>[4x]MDFLDSLIWERVVDDQYVTNPTFCISDYFEIVRQPGDGNCFYHSIAELFFDVKTPFSFRKVKEHLRLAADAFYDTEPEAIGTGVTKEEYIQAAMKDNEWGGSLEASMLSKQLQITIILWVVNQTEQVTAAIKFGPGRVSTALNLMHVGRTHFDALRVINQLEDNQLQSRSGSHHHHHH;>MATLNILVRNDKGRSSSYEVQLTQTVAVLKQQVCQRERVQADQFWLSFEGKPMDDEHPLGEYGLTTGCTVFMNLRLRG[4x]

Beyond the RNA-dependent RNA polymerase (RdRp), the L protein contains a viral homologue of the ovarian tumor domain protease (OTU) at the N-terminus. This OTU reverses posttranslational modifications by ubiquitin (Ub) and interferon (IFN) stimulated gene product 15 (ISG15). Sheep ISG15 was derivatized into a suicide inhibitor with propargylamine and incubated with KUPEV and GANV OTUs to form covalent complexes that could be used for X-ray crystallography. This yielded an atomic resolution structure of KUPEV OTU bound to the C-terminal domain of sheep ISG15 (C-sheep ISG15) solved to 2.06 Å and a low-resolution structure of GANV OTU bound to full length sheep ISG15 to 3.15 Å.

Examination of the high resolution KUPEV and low resolution GANV OTU-sheep ISG15 structures reveals them to possess the familiar overall mode of OTU-substrate binding, in which the OTU binds to the C-terminal domain of ISG15 by a mix of hydrophobic and electrostatic interactions. On the sheep ISG15 side, the interface with the OTUs is formed by W123, P130, and F149. One of the most noteworthy interactions is that of sheep ISG15 D89 forming water-mediated interactions with both KUPEV OTU T128 and R149. Interestingly, this results in D89 pointing away from the interface, contrasting with previous observations for this residue position in OTU-Ub structures and CCHFV OTU-human ISG15 structures. Considering the selectivity pocket in KUPEV is lined by hydrophobic residues V18, V120, A129, and I131, the adoption of a more solvent-exposed confirmation of the charged aspartate in sheep ISG15 is understandable. For instance, the OTUs from KUPEV and DUGV have limited activity for human proISG15, but efficiently cleave sheep and cow proISG15s and show moderate activity towards camel and vesper bat proISG15s. In the KUPEV OTU residue 122 is an asparagine residue, while CCHFV is unique among OTUs with an alanine at this position. As anticipated, the GANV OTU E122N mutant reduced activity for human ISG15-AMC almost 10-fold, while KUPEV OTU N122E boosted activity more than 6-fold relative to WT. In KUPEV OTU this residue is an isoleucine, creating the potential for a steric clash with the longer glutamate in human ISG15 compared to aspartate in sheep ISG15. In contrast, the KUPEV helix mutant (I80R/G81L/T82V) demonstrates a 5-fold increase in human ISG15-AMC activity while reducing Ub-AMC activity by half.>[2x]MDDANSSDSKVLNVWAMGDEAKSLKELAQKFTKDTGIEVKVQVIPWANAHDKLLTAVASKSGPDVVQMGTTWMPEFVEAGALLDITKDVEKSKNMNSDLFFPGS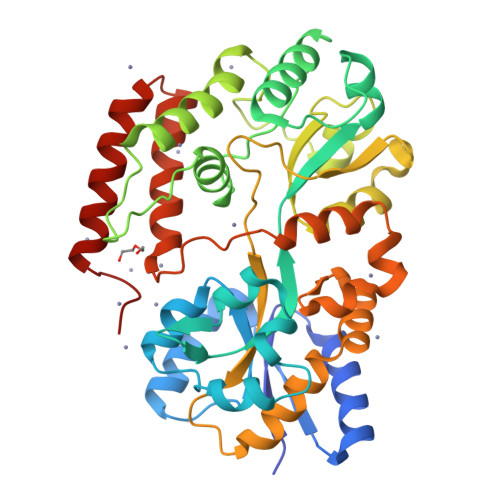VKTTQFDGKTYGVPWYAETRVLFYRTDLLKKVGYNEAPKTWDELSDAALKLSKRGKDMYGFAIDPNEQTTGFIFGRQNGSPLFDKDGTPVFNKKPFVDTVTYLDSFIKNGSAPDTDLGLDASQSFGGDGIVPMFMSGPWMVNTLKDTAPDIDGKWATAVLPKKENNESSLGGANLSIFKYSNKKDDALKFMDYMSQPDVQLSWLKDTNSMPARMDAWEDDMLKNDPYYKVFGEQMKTAEPMPLIPQFEEIAQLYGKSWEQIYRGGADVQTQMDTFNDQVEALLKKLEHHHHHH>[2x]GAKPYEKVRIYRMDGSYRSVELKHGNNTTVQQIMEGMRLSQETQQYFTIWICSENLSLQLKPYHKPLQHVRDWPEILAELTNLDPQRETPQLFLRRDVRLPLEVEKQIEDPLAILILFDEARYNLLKGFYTAPDAKLITLASLLL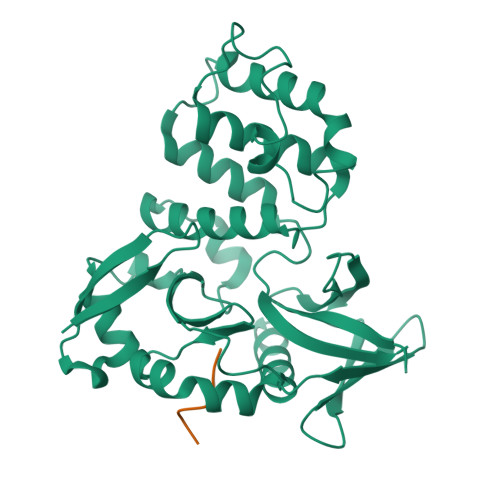QIVYGNYESKKHKQGFLNEENLKSIVPVTKLKSKAPHWTNRILHEYKNLSTSEGVSKEMHHLQRMFLQNCWEIPTYGAAFFTGQIFTKASPSNHKVIPVYVGVNIKGLHLLNMETKALLISLKYGCFMWQLGDTDTCFQIHSMENKMSFIVHTKQAGLVVKLLMKLNGQLMPTERNS;>SRHSCIFPGQYNPSFISDESRRRDYF[2x]> PPRKASKASLDFKRYVTDRRLAETLAQIYLGKPSRPPHLLLECNPGPGILTQALLEAGAKVVALESDKTFIPHLESLGKNLDGKLRVIHCDFFKLDPRSGGVIKPPAMSSRGLFKNLGIEAVPWTADIPLKVVGMFPSRGEKRALWKLAYDLYSCTSIYKFGRIEVNMFIGEKEFQKLMADPGNPDLYHVLSVIWQLACEIKVLHMEPWSSFDIYTRKGPLENPKRRELLDQ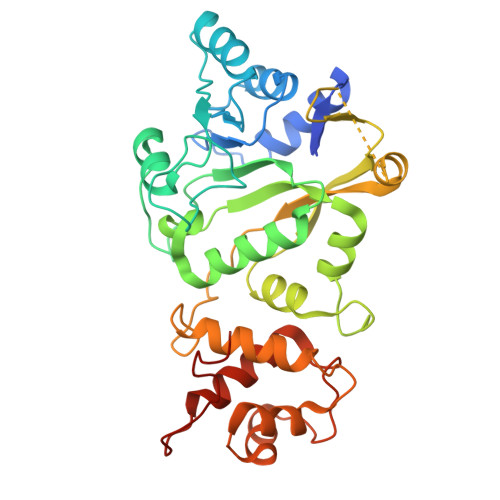LQQKLYLIQMIPRQNLFTKNLTPMNYNIFFHLLKHCFGRRSATVIDHLRSLTPLDARDILMQIGKQEDEKVVNMHPQDFKTLFETIERSKDCAYKWLYDETLEDR> MSSSFVSNGASLEDCHCNLFCLADLTGIKWKRYVWQGPTSAPILFPVTEEDPILSSFSRCLKADVLGVWRRDQRPGRRELWIFWWGKDPNFADLIHHDLSEEEDGVWENGLSYECRTLLFKAVHNLLERCLMNRNFVRIGKWFVKPYEKDEKPINKSEHLSCSFTFFLHGDSNVCTSVEINQHQPVYLLSEEHVTLAQQSNSPFQVILSPFGLNGTLTGQAFKMSDSATKKLIGEWKQFYPISCGLKEMSEEKQDDMDWEDDSLAAVEVLVAGVRMIYPACFVLVPQSDIPAPSSVGASHCSASCLGIHQVPASTRDPAMSSVTLTPPTSPEEVQTVDPQSAQKWVKFSSVSDGFSTDSTSHHGGKIPRKLANHVVDRVWQECNMNRLQNKRKYSATSSGLCEEETADKIGCWDFVEATQRTSCSCLRHKSLKTRNTGQQGQAPSLGQQQQVLPKHKTNEKQDKSEKPQKRPLTPFHHRVSVSDEIGMDTDSASQRLVISAADSQVRFSNIRTNDVAKTPQMHGTELANSPQPPPLSPHPCDVVDEGVTKTPSTPQSQHFYQMPTPDPLVPTKPMEDRIDSLSQSFPPPFQEAVEPTVYVGTAVSLEEDEANVAWKYYKVPKKKDVEFLPPQLPNDKFKDDPVGPFGQESVTSVTELMVQCKKPLKVSDEIVQQYQIKNQYLSAIASDTEQEPKIDPYAFVEGDEEFIFTDKKDRQNSEREAGKKHKVEDGTSAVTVLSHEEDAMSLFSPSKQDAPRPTNHARPPSTSLIYDSDLAVSYTDLDNLFNSDEDELTPGSKKSASGSDDKASSKESKTGNLDPLSCISTADLHKMYPTPPSLEQHIMGFSPMNMNNKEYGSVDTAPGGTVLEGNSSSVGTQFRIEVEEGFCSPKPSEIKDFSYVYKPENCQVLVGCSMFAPLKTLPSHCLPPIKLPEECVYRQSWTVGKLDLLPSGPSMPFIKEGDGSNLDQDYGPAYTPQTHASFGMPPSSAPPSNGGAGILPSPSTPRFPTPRTPRTPRTPRGAGGPASAQGSVKYENSDLYSPASTPSTCRPLNSVEPATVPSIPEAHSLYVNLILSESVMNLFKDCNFDSCCICVCNMNIKGADVGVYIPDPTQEAQYRCTCGFSAVMNRKFGNNSGLFLEDELDIIGRNTDCGKEAEKRFEALRASSVENVNGGLKESEKVPDELILLLQDQCTNLFSPFGAADQDPFPKVGISSNWVRVEERDCCSDCCLALEHGRQFMDNMSGGKVDEALVRSSCLHPWAKQNDASVQCSQDILRMLLSLQPVLQDAIQKKRTVRPWGVQGPLTWQQFHKMAGRGSYGTDESPEPLPIPTFLLGYDYDFLVLSPFALPYWEKLMLEPYGSQRDIAYVVLCPENEALLNGARSFFRDLTAIYESCRLGQHRPISRLLTDGIMKVGATASKKLSEKFVTEWFSQAADGNNEAFSKLKLYAQVCRYDLGPYLASQPLDSSLLSQPNLVAPPNQSLVTAPQMTNTGNANAPSATLASAASSTMTMTSGVPISTSVATANSTLTTTSSSSSSSLSSGVSSNKLPSFPPFGSMN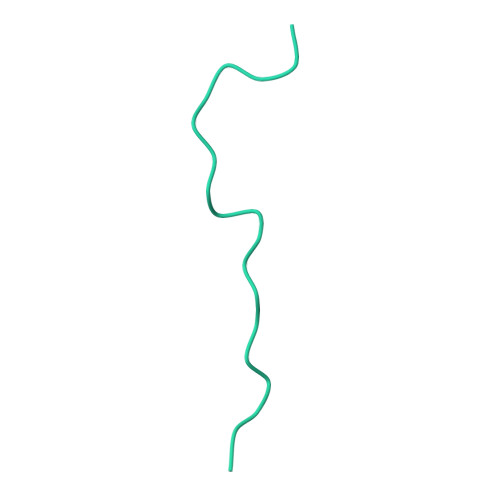TSGTGSMSAQASTVQSGQLGGQQSSSLQAAGISGESASLPTQPHPDVSESTMDRDKVGIPTDGDSHAITYPPAIVVYIIDPFTYENKDESTNSSNVWTLGLLRCFLEMVQTLPPHIKSTVSVQIVPCQYLLQPVKHDDRQIYSQHLKSLAFSVFTQCRRPLPTSTNVKTLTGFGPGLAMETALKSPDRPECIRLYTPPFILAPVKDKQTELGETFGEAGQKYNVLFVGYCLSHDQRWILASCTDLYGELLETCIINIDVPNRARRKKGSARRFGLQKLWEWCLGLVQMSSLPWRVVIGRLGRIGHGELKDWSCLLSRRNLQSLSKRLKDMCRMCGISAADSPSILSACLVAMEPQGSFVIMPDSVSTGSVFGRSTTLNMQTPQLNTPQDTSCTHILVFPTSASVQVASATYTTENLDLAFNPNNDGADGMGIFDLLDTGDDLDPDIINILPASPTASPVHSPGSHYPHGGDAGKGQGTDRLLSTESHDEVTNILQQPLALGYFVSTAKAGPLPDWFWSACPQAQYQCPLFLKASLHLHVPSVQSDELLHSKHSHPLDSNQTSDVLRFVLEQYNALSWLTCDPAVQDRRSCLPVHFVVLNQLYNFIMNML Survival of motor neuron (SMN) functions in diverse biological pathways via recognition of symmetric dimethylarginine (Rme2s) on proteins by its Tudor domain, and deficiency of SMN leads to spinal muscular atrophy. Here we report a potent and selective antagonist with a 4-iminopyridine scaffold targeting the Tudor domain of SMN. In order to understand the structural basis of compound 1 recognition by these reader proteins, we determined the crystal structures of compound 1 in complex with SMN, TDRD3 and UHRF1, respectively. In this study, we identified some low micromolar antagonists with a 4-iminopyridine scaffold targeting the Tudor domain of SMN, and compound 1 shows >4-fold selectivity over other tested methyllysine or methylarginine binding domains.

In addition to triple-ring compounds 1 to 4, SMN also bound to two of twelve double-ring compounds, compounds 5 and 6. Both compounds retain the imino group, which pinpoints the importance of the imino group-mediated hydrogen bond in the compound binding and is consistent with our crystal structures of SMN in complex with compounds 1, 4, and 6. None of the single-ring compounds bound to SMN, which may not be able to provide strong enough π–π stacking interaction to hold the compounds.

>KKNTAASLQQWKVGDKCSAIWSEDGCIYPATIASIDFKRETCVVVYTGYGNREEQNLSDLLSPICE[4x]> MTQELGNANFENFIGATEGFSEIAYQFTSHILTLGYAVMLAGLLYFILTIKNVDKKFQMSNILSAVVMVSAFLLLYAQAQNWTSSFTFNEEVGRYFLDPSGDLFNNGYRYLNWLIDVPMLLFQILFVVSLTTSKFSSVRNQFWFSGAMMIITGYIGQFYE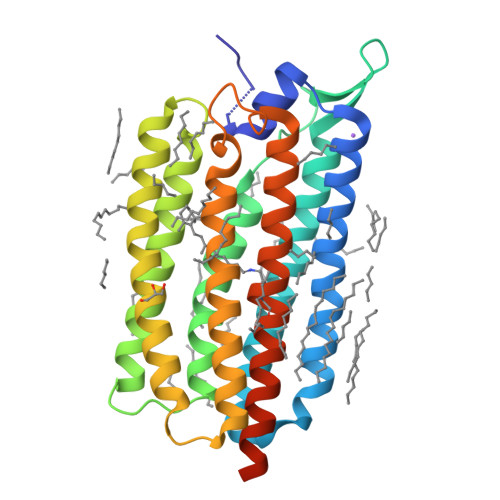VSNLTAFLVWGAISSAFFFHILWVMKKVINEGKEGISPAGQKILSNIWILFLISWTLYPGAYLMPYLTGVDGFLYSEDGVMARQLVYTIADVSSKVIYGVLLGNLAITLSKNKELVEANSLEHHHHHH> MITSALHRAADWAKSVFSSAALGDPRRTARLVNVAAQLAKYSGKSITISSEGSKAAQEGAYRFIRNPNVSAEAIRKAGAMQTVKLAQEFPELLAIEDTTSLS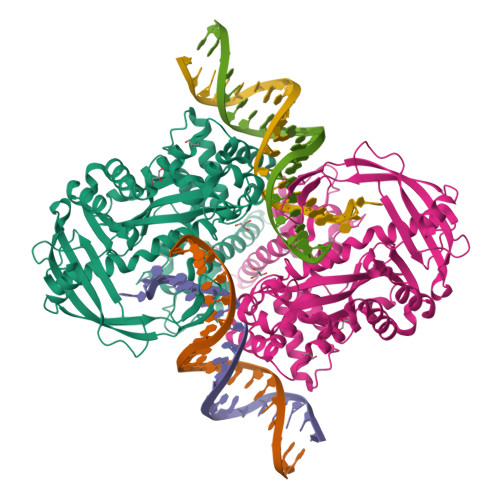YRHQVAEELGKLGSIQDKSRGWWVHSVLLLEATTFRTVGLLHQEWWMRPDDPADADEKESGKWLAAAATSRLRMGSMMSNVIAVCDREADIHAYLQDKLAHNERFVVRSKHPRKDVESGLYLYDHLKNQPELGGYQISIPQKGVVDKRGKRKNRPARKASLSLRSGRITLKQGNITLNAVLAEEINPPKGETPLKWLLLTSEPVESLAQALRVIDIYTHRWRIEEFHKAWKTGAGAERQRMEEPDNLERMVSILSFVAVRLLQLRESFTPPQALRAQGLLKEAEHVESQSAETVLTPDECQLLGYLDKGKRKRKEKAGSLQWAYMAIARLGGFMDSKRTGIASWGALWEGWEALQSKLDGFLAAKDLMAQGIKIG>[2x]NYKKPKLLYCSNGGHFLRILPDGTVDGTRDRSDQHIQLQLSAESVGEVYIKSTETGQYLAMDTDGLLYGSQTPNEECLFLERLEENHYNTYISKKHAEKNWFVGLKKNGSCKRGPRTHYGQKAILFLPLPVSSD;>TDNTKPNRMPVAPYWTSPEKMEKKLHAVPAAKTVKFKCPSSGTPNPTLRWLKNGKEFKPDHRIGGYKVRYATWSIIMDSVVPSDK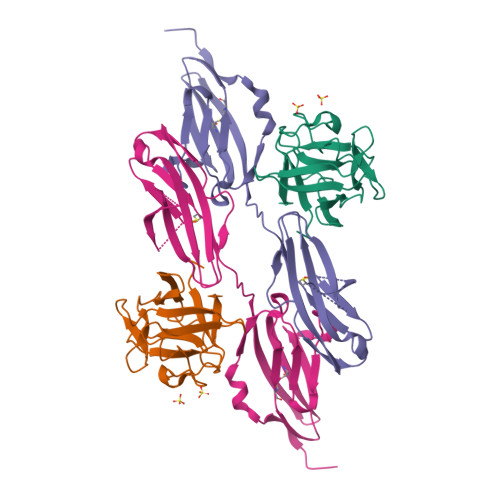GNYTCIVENEYGSINHTYQLDVVERSPHRPILQAGLPANKTVALGSNVEFMCKVYSDPQPHIQWLKHIEVNGSKIGPDNLPYVQILKTAGVNTTDKEMEVLHLRNVSFEDAGEYTCLAGNSIGLSHHSAWLTVLEALEER[2x]>[4x]SSVPPTPEERHMLLNGDWIRYYHFYPM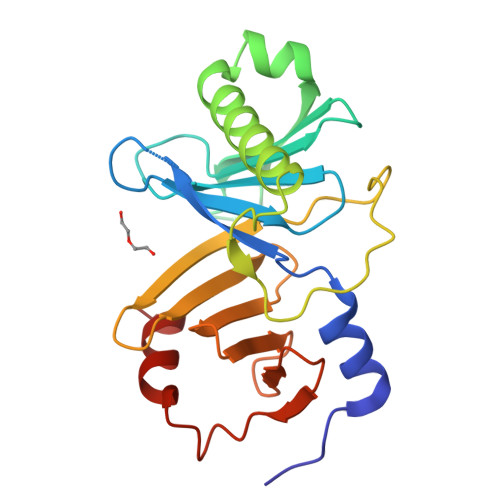EEEGGDSVAVTYHIQPGRTGVTFFNHSFSVHSAVLSVLEHIVYVVDRVDIEEDNDVARILSLAQALNEEKKIYDVLQLVETHDTHMLKQRRSPGIMSVYCPPQTAFQCNGDPFVFVRWYRFHMENSMSGFMLSNGAVQVFVGGKYELRWLDDNRKFIVRSNGVCEVLDEEKFPLSEELNQMLYGGV> MFVARSIAADHKDLIHDVSFDFHGRRMATCSSDQSVKVWDKSESGDWHCTASWKTHSGSVWRVTWAHPEFGQVLASCSFDRTAAVWEEIVGESNDKLRGQSHWVKRTTLVDSRTSVTDVKFAPKHMGLMLATCSADGIVRIYEAPDVMNLSQWSLQHEISCKLSCSCISWNPSSSRAHSPMIAVGSDDSSPNAMAKVQIFEYNENTRKY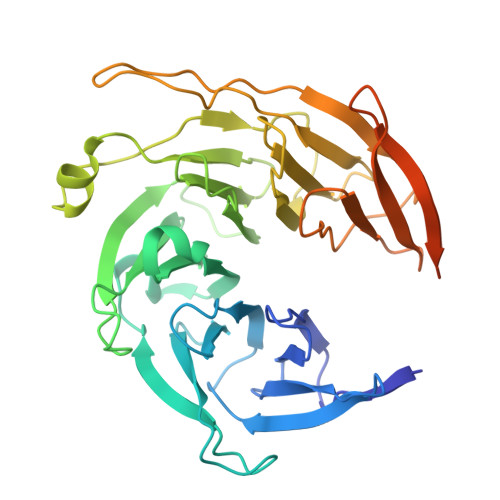AKAETLMTVTDPVHDIAFAPNLGRSFHILAIATKDVRIFTLKPVRKELTSSGGPTKFEIHIVAQFDNHNSQVWRVSWNITGTVLASSGDDGCVRLWKANYMDNWKCTGILKGNGSPVNGSSQQGTSNPSLGSTIPSLQNSLNGSSAGRKHS6-[[2-[1-(6-methoxy-1,5-naphthyridin-4-yl)-1,2,3-triazol-4-yl]ethylamino]methyl]-4H-1,4-benzothiazin-3-one 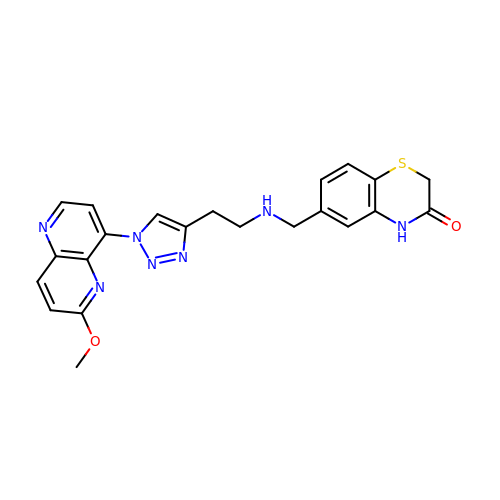| C22 H21 N7 O2 S | IFTKOVLUZDBNBQ-UHFFFAOYSA-N> MFKQIPLGPIQTNAYVLYNDDKEAVIFDPGGDAEALITWLKREQLTPLAILLTHAHFDHIGAVDAVRDTFSIPVYLHTKERHWLEDPALNGSSRLTGRPITTAKPADHLLTNEKSLTIGTFTFSVFHTPGHSPGSVSYYYQKEAVLFSGDVLFQQSIGRTDLRGGDHTLLLA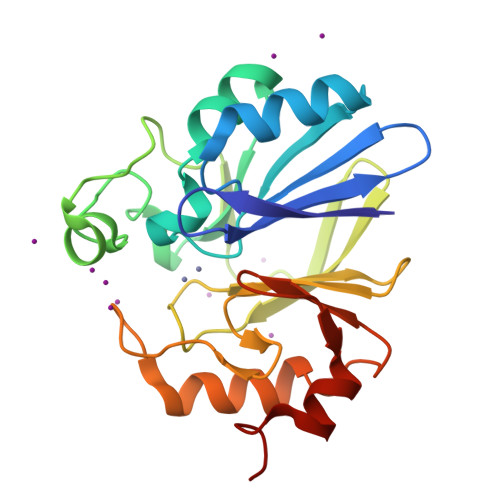SIHNKILPLPERTIVASGHGPLTTIGQEMDHNPFLTGY> MSNKVKTKAMVPPINCIFNFLQQQTPVTIWLFEQIGIRIKGKIVGFDEFMNVVIDEAVEIPVNSADGKEDV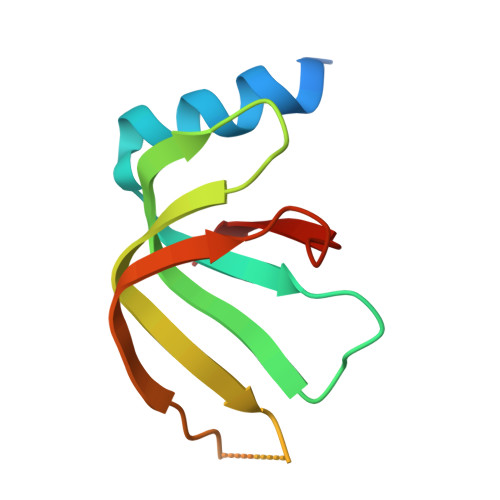EKGTPLGKILLKGDNITLITSAD>S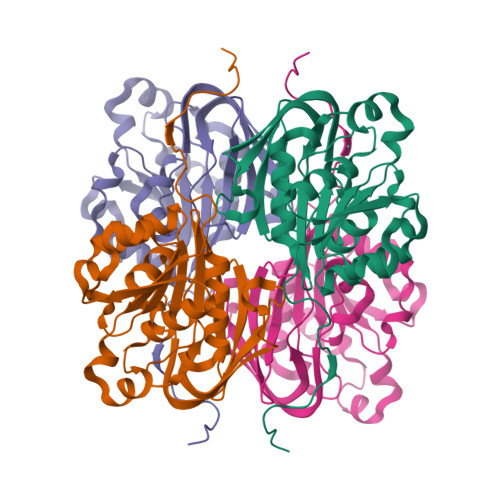NAMTTPIRVVVWNEFRHEKKDEQVRAIYPEGMHTVIASYLAEAGFDAATAVLDEPEHGLTDEVLDRCDVLVWWGHIAHDEVKDEVVERVHRRVLEGMGLIVLHSGHFSKIFKKLMGTTCNLKWREADEKERLWVVAPGHPIVEGIGPYIELEQEEMYGEFFDIPEPDETIFISWFEGGEVFRSGCTFTRGKGKIFYFRPGHETYPTYHHPDVLKVIANAVRWAAPVNRGEIVFGNVKPLEPIKAKQGGVTQ[8x]>[4x]SNAMDFKLE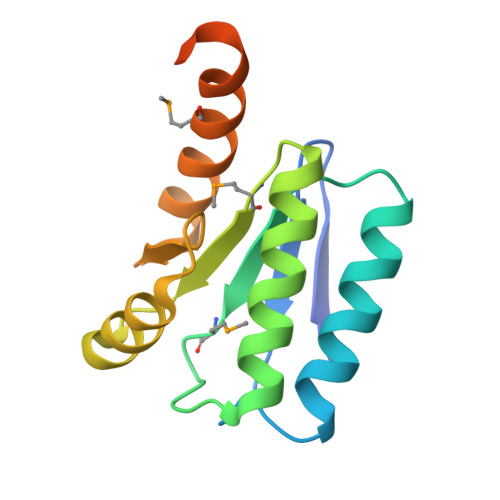KKEQYVYIETDAPAFAGDVPAAFEETARSLFREGYHSLIVNMQTVKSLDATGITTLKKVNYLCANDLGMLAIVTRDDDFIDLLEDLRIPDLTVLPTKEEAIDAVFMHSLENEFGAGDDDYDDEDYEGVSESKEP> GSLLPRLPSEPGMTLLTLTIEKIGLKDAGQCIDPYITVSVKDLNGIDLNPVQDTPVATRKEDTYIHFSVDVEIQRHLEKLPKGAAIFFEFKHYKPKKRFTSTKCFAFMEMDEIKPGPIVIELYKKPTDFKRKKLNLLTKK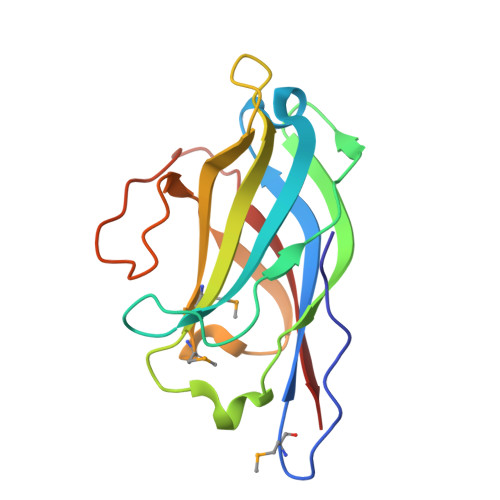PLYLHLNQTLHK> MNNNKAEADTSSSMADPETRPTYTTHHLAIPSGVTQDEFDELKQSVVEFHTYQLSQNQCSSLLAQRIRAPNDVVWSIVRRFDQPQTYKHFIKSCSVSDNFTMAVGSTRDVNLISGLPAATSTERLDILDDDRQVLGISIIGGEHRLRNYRSVISVHGFNRDGAICTVALESYVVDVPEGNTEEDTRLFADTVVKLNLQKLVSVAESQVI;> RSVYELDCIPLWGTVSIQGNRSEMEDAFAVSPHFLKLPIKMLMGDHEGESPSLTHLTGHFFGVYDGHGGHKVADYCRDRLHFALAEEIERIKDELCKRNTGEGRQVQWDKVFTSCFLTVDGEIEGKIGRAVVGSSDKVLEAVASETVGSTAVVALVCSSHIVVSNCGDSRAVLFRGKEAMPLSVDHKPDREDEYARIENAGGKVIQWQGARVFGVLAMSRSIGDRYLKPYVIPEPEVTFMPRSREDECLILASDGLWDVMNNQEVCEIARRRILMWHKKNGAPPLAERGKGIDPACQAAADYLSMLALQKGSKDNISIIVIDLKAQRKFKTRT

Enhanced ABA levels elicited in response to drought are perceived by the PYR/PYL/RCAR family of ABA receptors and the clade A subfamily of protein phosphatases type 2C (PP2Cs), which act as necessary ABA co-receptors in ternary complexes. In the resting state, PYLR/PYL/RCAR receptors display an open ABA binding cavity flanked by two highly conserved loops, named as gate/CL2/β3-β4 loop and latch/CL3/β5-β6 loop. Specifically, both gate and latch loops define a surface that enables the receptor to dock into the PP2C active site. The formation of receptor-ABA-phosphatase complexes causes the dissociation of different PP2C-SnRK2 complexes and abolishes PP2C-mediated inhibition of the SnRK2s, triggering ABA response.

Using a structure-guided approach, we have engineered a Citrus sinensis PYL1 (CsPYL1) variant, named CsPYL15m, which shows enhanced affinity for SB. We observed increased sensitivity to SB of CsPYL15m with respect to the WT as the IC50 of SB was 12-fold lower for the synthetic receptor. The comparison of CsPYL1 and CsPYL5m binding pockets reveals that CsPYL15m displays a closer interaction with SB at mutated Leu112, whose methyl groups show favorable contacts with the SB’s aromatic bicyclic ring (middle and right). In addition, an enlargement of the binding pocket at Ile137 is observed (right). This free space is filled with water molecules that interact with the polar side chain of Lys88, which is otherwise buried in a more hydrophobic environment in the WT receptor bound to SB (right). Thus, Lys88 of CsPYL15m is more amenable to polar interactions in the pocket of CsPYL15m bound to SB. Together, these structural insights may explain the enhanced sensitivity of CsPYL15m to SB. Recently, opabactin has been described as a powerful ABA agonist and a key feature for its enhanced interaction with ABA receptors in the presence of a carboxylate group that interacts with a conserved Lys residue in the ABA binding pocket. Both CsPYL1-SB-HAB1 and CsPYL15m-SB-HAB1 complexes lack such interaction of the agonist with the conserved Lys88 residue of the receptor; rather, the structures show that the hydrophobic CH2 of the SB linker faces a water-filled cavity harboring the side-chain NH3+ of Lys88 (middle and right).CDT is a member of the Iota family of protein toxins which also consists of two homologous toxins produced by Clostridium perfringens (the Iota toxin) and Clostridium spiroforme (C. spiroforme Transferase, CST). All three Iota toxin family members are assembled from two polypeptide chains termed the “A” subunit (CDTa, Ia, and CSTa) and “B”, subunit (CDTb, Ib, and CSTb). All three B subunits are presumed to contain five domains that are involved in regulation (D1), oligomerization (D2 and D3), and host recognition (D3’ and D4). Once proteolyzed, the mature form of CDTb forms a large heptameric, soluble structure referred to as the prepore which binds one molecule of CDTa to generate the toxic moiety, CDT.

Still, maps of modest global resolution could be reconstructed for the CDTb dimer (3.74 Å), trimer (4.08 Å), tetramer (4.08 Å), and symmetric heptamer (3.27 Å) which enabled map refinement and model construction. Similarly, the number of symmetric particles in this dataset were not equal, with the heptameric structure ~44-fold more abundant than the octameric form. Although the unique pathway we describe for CDT also results in the formation of heptameric and octameric structures, the octameric structures are present at a significantly lower abundance in vitro when compared to that observed for anthrax toxin in a cellular model (~1.5% and ~30% in CDT and anthrax toxin, respectively). Conversely, the particles isolated in fraction five retained a high molecular weight, suggesting the symmetric heptamer does not spontaneously disassemble upon dilution. Indeed, residues 456–463 of CDTb remain unengaged and dynamic in the structures we describe here but interface in the symmetric heptamer. Our observation that small oligomeric intermediates, but not the assembled symmetric structures, spontaneously assemble and disassemble would support this hypothesis.

>[7x]MKIQMRNKKVLSFLTLTAIVSQALVYPVYAQTSTSNHSNKKKEIVNEDILPNNGLMGYYFTDEHFKDLKLMAPIKDGNLKFEEKKVDKLLDKDKSDVKSIRWTGRIIPSKDGEYTLSTDRDDVLMQVNTESTISNTLKVNMKKGKEYKVRIELQDKNLGSIDNLSSPNLYWELDGMKKIIPEENLFLRDYSNIEKDDPFIPNNNFFDPKLMSDWEDEDLDTDNDNIPDSYERNGYTIKDLIAVKWEDSFAEQGYKKYVSNYLESNTAGDPYTDYEKASGSFDKAIKTEARDPLVAAYPIVGVGMEKLIISTNEHASTDQGKTVSRATTNSKTESNTAGVSVNVGYQNGFTANVTTNYSHTTDNSTAVQDSNGESWNTGLSINKGESAYINANVRYYNTGTAPMYKVTPTTNLVLDGDTLSTIKAQENQIGNNLSPGDTYPKKGLSPLALNTMDQFSSRLIPINYDQLKKLDAGKQIKLETTQVSGNFGTKNSSGQIVTEGNSWSDYISQIDSISASIILDTENESYERRVTAKNLQDPEDKTPELTIGEAIEKAFGATKKDGLLYFNDIPIDESCVELIFDDNTANKIKDSLKTLSDKKIYNVKLERGMNILIKTPTYFTNFDDYNNYPSTWSNVNTTNQDGLQGSANKLNGETKIKIPMSELKPYKRYVFSGYSKDPLTSNSIIVKIKAKEEKTDYLVPEQGYTKFSYEFETTEKDSSNIEITLIGSGTTYLDNLSITELNSTPEILDEPEVKIPTDQEIMDAHKIYFADLNFNPSTGNTYINGMYFAPTQTNKEALDYIQKYRVEATLQYSGFKDIGTKDKEMRNYLGDPNQPKTNYVNLRSYFTGGENIMTYKKLRIYAITPDDRELLVLSVD>MATHHTLWMGLALL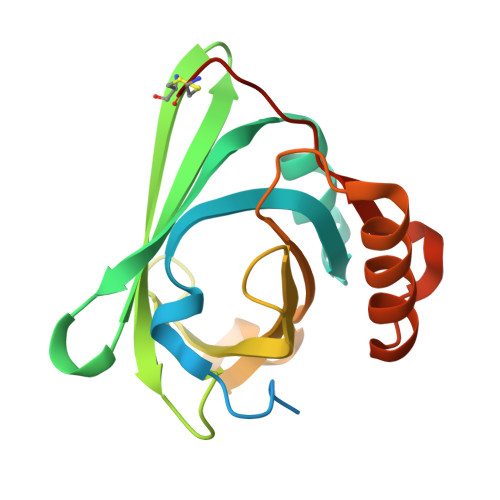GVLGDLQAAPEAQVSVQPNFQQDKFLGRWFSAGLASNSSWLREKAAALSMAKSVVAPATDGGLNLTSTFLRKNQCETRTMLLQPAGSLGSYSYRSPHWGSTYSVSVVETDYDQYALLYSQGSKGPGEDFRMATLYSRTQTPRAELKEKFTAFCKAQGFTEDTIVFLPQTDKCMTEQ[8x]The KPC β-lactamases present a larger and more ominous global threat. Boronic acid transition state inhibitors (BATSIs) are competitive, reversible BLIs that offer promise as novel therapeutic agents. Boronic acid transition state inhibitors (BATSIs) have the potential to become clinically important BLIs, which would add to the success of FDA-approved vaborbactam, as they possess a boron atom acting as an electrophile that mimics the carbonyl carbon of the β-lactam ring and forms a tetrahedral adduct with the catalytic serine that closely resembles the transition state in the hydrolytic mechanism. In this study, the activities of two α-amido-β-triazolylethaneboronic acid transition state inhibitors (S02030 and MB_076) targeting representative KPC (KPC-2) and CTX-M (CTX-M-96, a CTX-M-15-type extended-spectrum β-lactamase [ESBL]) β-lactamases were evaluated.

MB_076 was designed to improve oxidation stability and hydrophobic interactions in the active site of serine class A β-lactamases, replacing the thiophene ring of S02030 with an amino-thiadiazole ring. A crystal structure of KPC-2 with MB_076 bound was solved at 1.38 Å resolution. The unbiased omit map contoured at 2.5 σ revealed density for MB_076 being covalently attached to the Oγ atom of the catalytic S70 residue. MB_076 was refined to an occupancy of 0.8. The two boronic acid hydroxyls of MB_076 form stabilizing interactions and occupy the oxyanion hole (formed by backbone N:H exchangers [NHEs] of S70 and T237) and the deacylation water pocket (formed by E166 and N170) of KPC-2. The carboxylate binding group of the MB_076 is situated in the β-lactam carboxyl binding pocket and forms hydrogen bonds in the active site with S130, T235, and T237. The carbonyl oxygen in MB_076 interacts and forms a hydrogen bond with N132. The C-H of the triazole ring is polar and can form a 3.0-Å C-H—O hydrogen bond interaction with the hydroxyl of S130. In accordance with our goal (to improve hydrophobic interactions by its thiophene ring) the CH2-S-thiadiazole ring-containing portion of MB_076 engages in hydrophobic interactions with N170, the main chain atoms of C238, and T237. Furthermore, the amino-thiadiazole ring forms intramolecular edge-to-face π-π interactions with the triazolyl moiety of MB_076.

> ALTNLVAEPFAKLEQDFGGSIGVYAMDTGSGATVSYRAEERFPLCSSFKGFLAAAVLARSQQQAGLLDTPIRYGKNALVPWSPISEKYLTTGMTVAELSAAAVQYSDNAAANLLLKELGGPAGLTAFMRSIGDTTFRLDRWELELNSAIPGDARDTSSPRAVTESLQKLTLGSALAAPQRQQFVDWLKGNTTGNHRIRAAVPADWAVGDKTGTCGVYGTANDYAVVWPTGRAPIVLAVYTRAPNKDDKHSEAVIAAAARLALEGLG> MKELIYIEEPSILFAHGQKCTDPRDGLALFGPLNQIYGIKSGVVGTQKGLQIFKSY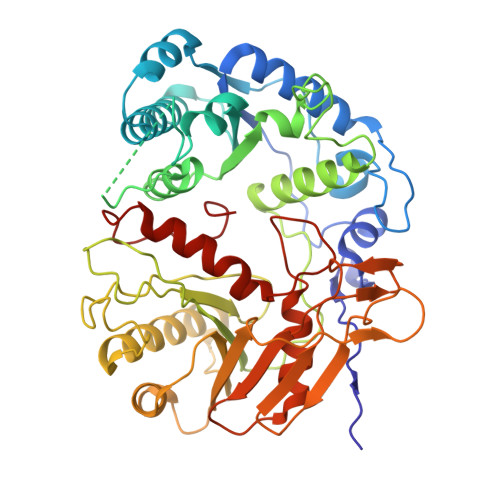LDKIQKPIYNHNNITRPMFPGFEAVFGCKWESQNIVFKEITDEEIRRYLFNASTHKRTYDLVTLFNDKIITANKNDEERVDVWFVIVPEEIYKYCRPNSVLPNELVQTKSLISKSKAKSFRYTPTLFEEFNKKLKEVEKEAKTYNYDAQFHDQLKARLLEHTIPTQILRESTLAWRDFKNTFGAPIRDFSKIEGHLAWTISTAAYYKAGGKPWKLGDIRPGVCYLGLVYKKIEKSKNPQNACCAAQMFLDNGDGTVFKGEVGPWYNPEKGEYHLKPKEAKALLTQALESYKEQNKSYPKEVFIHARTRFNDEEWNAFNEVTPKNTNLVGVTITKSKPLKLYKTEGAFPIMRGNAYIVDEKKAFLWTLGFVPKLQSTLSMEVPNPIFIEINKGEAEIQQVLKDILALTKLNYNACIYADGEPVTLRFANKIGEILTASTEIKTPPLAFKYYI>SMRAKKMGTVRPWATGLSGQLQKAFVTGVPSLKRSELETACEDFSNIIGSTSTCMLYKGTLSSGVEIAVASSLVTSAKDWSKENESQYRKKITNLSKVSHKNFMNLLGYCEEEHPFT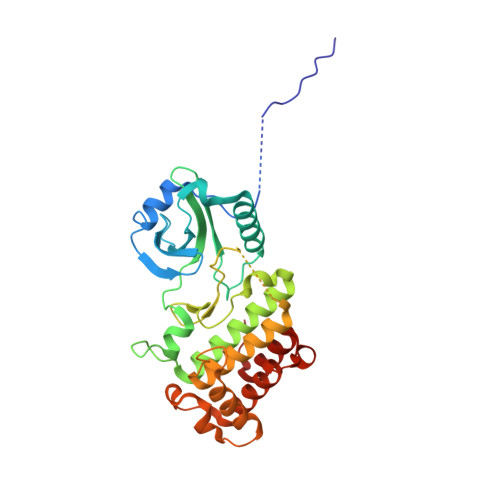RVMVFEYAPNGTLFEHLHVREAEKLDWMARLRISMGIAYCLEHMHQLQTPAALRNFDSTTVYLTDDFAAKVSDLEFWNDAKGHNSTTNNELAFSPDMEDIVRKYGMVLLEILTGRVPSSEDDGPLENWVSRYFEGGMRLEELIDPSIGFFPEDTARALCEVVRSCIDRDPKKRPQMKEVAARMREITALGP[2x]>AEKNYVMAIDQGTTSSRAIIFDRNGKKIGSSQKEFPQYFPKSGWVEHNANEIWNSVQSVIAGAFIESGIRPEAIAGIGITNQRETTVVWDKTTGQPIANAIVWQSRQSSPIADQLKVDGHTEMIHEKTGLVIDAYFSATKVRWLLDNIEGAQEKADNGELLFGTIDSWLVWKLTDGQVHVTDYSNASRTMLYNIHKLEWDQEILDLLNIPSSMLPEVKSNSEVYGHTRSYHFYGSEVPIAGMAGDQQAALFGQMAFEKGMIKNTYGTGAFIVMNTGEEPQLSDNDLLTTIGYGINGKVYYALEGSIFVAGSAIQWLRDGLRMIETSPQSEELAAKAKGDNEVYVVPAFTGLGA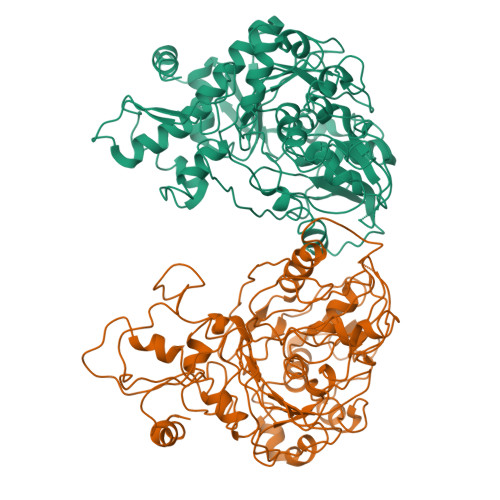PYWDSEARGAVFGLTRGTTKEDFVRATLQAVAYQSKDVIDTMKKDSGIDIPLLKVDGGAAKNDLLMQFQADILDIDVQRAANLETTALGAAYLAGLAVGFWKDLDELKSMAEEGQMFTPEMPAEERDNLYEGWKQAVAATQTFKFKAKKEGE[2x]>[2x]SNAMAASDQHRSRRHDESSSRPNKKKKVSRNPETNLLFNLNSCSKSKDLSAALALYDAAITSSEVRLSQQHFQTLLYLCSASITDISLQYLAIDRGFEIFDRMVSSGISPNEASVTSVARLAAAKGNGDYAFKVVKEFVSVGGVSIPRLRTYAPALLCFCEKLEAEKGYEVEEHMEAAGIALEEAEISALLKVSAATGRENKVYRYLHKLREYVGCVSEETLKIIEEWFCGEKAGEVGDNGIGSDVG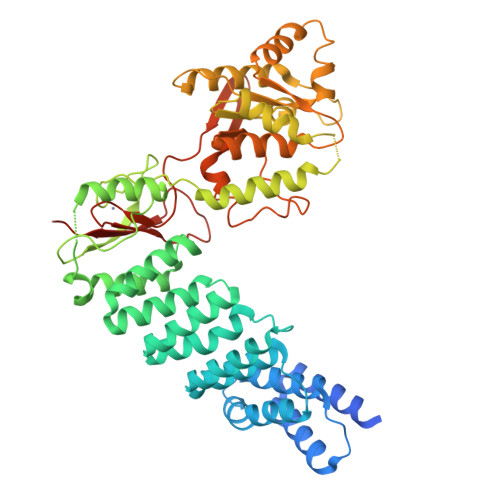MLREAVLNNGGGWHGHGWVGEGKWTVKKGNVSSTGRCLSCSEQLACVDTNEVETQKFVDSLVALAMDRKTKMNSCETNVVFSEFQDWLEKHGDYEAIVDGANIGLYQQNFVDGSFSLSQLESVMKELYRESGNNKWPLILLHKRRVKTLLENPTHRNLVEEWISNGVLYATPPGSNDDWYWLYAAAKLKCLLVTNDEMRDHIFELLGSTFFQKWKERHQVRYTFVKGNLKLEMPSPFSVVIQESEKGSWHFPVSCENNEESSRTWMCISRQSILDSPKSNGKIP>MSFSSKPTVLASRVESDSAINVMKWKT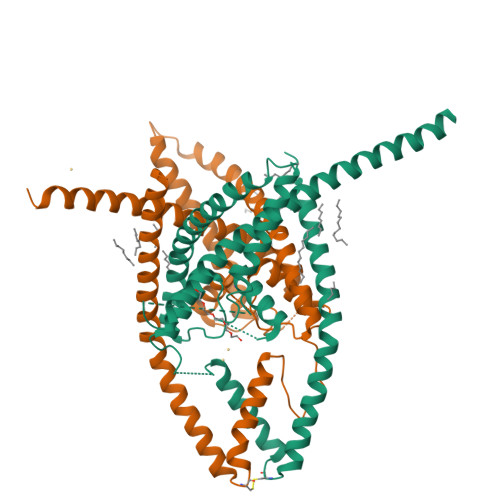VSTIFLVVVLYLIIGATVFKALEQPQEISQRTTIVIQREKFLRAHPCVSDQELDELIQQIVAAINAGIIPLGASSNQVSHWDLGSSFFFAGTVITTIGFGNISPRTEGGKIFCIIYALLGIPLFGFLLAGVGDQLGTIFGKGIAKVEDTFIKWNVSQTKIRIISTIIFILFGCVLFVALPAVIFKHIEGWSALDAIYFVVITLTTIGFGDYVAGGSDIEYLDFYKPVVWFWILVGLAYFAAVLSMIGDWLRVIAKKTKEAVGEFRAHAAEWTANVTSNSLEVLFQ[2x]>[2x]ADKELKFLVVDDFSTMRRIVRNLLKELGFNNVEEAEDGVDALNKLQAGGYGFVIS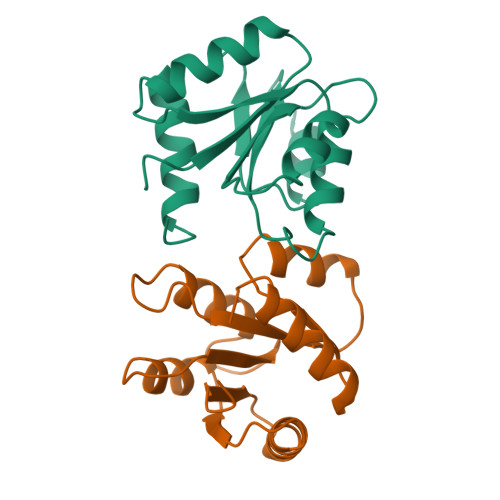DWNMPNMDGLELLKTIRADGAMSALPVLMVIAEAKKENIIAAAQAGASGYVVKPFTAATLEEKLNKIFEKLGM>[2x]MEGSEPVAAHQGEEASCSSWGTGSTNKNLPIMSTASVEIDDALYSRQRYVLGDTAMQKMAKSHVFLSGMGGLGLEIAKNLVLAGIKAVTIHDTEKCQAWDLGTNFFLSEDDVVNKRNRAEAVLKHIAELNPYVHVTSSSVPFNETTDLSFLDKYQCVVLTEMKLPLQKKINDFCRSQCPPIKFISADVHGIWSRLFCDFGDEFEVLDTTGEEPKEIFISNITQANPGIVTCLENHPHKLETGQFLTFREINGMTGLNGSIQQITVISPFSFSIGDTTELEPYLHGGIAVQVKTPKTVFFESLERQLKHPKCLIVDFSNPEAPLEIHTAMLALDQFQEKYSRKPNVGCQQDSEELLKLATSISETLEEKPDVNADIVHWLSWTAQGFLSPLAAAVGGVASQEVLKAVTGKFSPLCQWLYLEAADIVESLGKPECEEFLPRGDRYDALR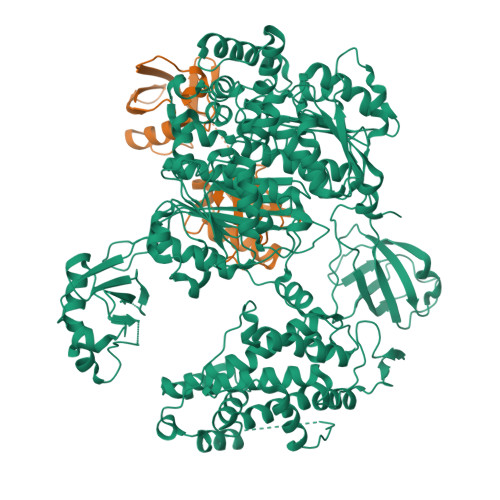ACIGDTLCQKLQNLNIFLVGCGAIGCEMLKNFALLGVGTSKEKGMITVTDPDLIEKSNLNRQFLFRPHHIQKPKSYTAADATLKINSQIKIDAHLNKVCPTTETIYNDEFYTKQDVIITALDNVEARRYVDSRCLANLRPLLDSGTMGTKGHTEVIVPHLTESYNSHRDPPEEEIPIATLKNFPNAIEHTLQWARDEFEGLFKQPAENVNQYLTDPKFVERTLRLAGTQPLEVLEAVQRSLVLQRPQTWADCVTWACHHWHTQYSNNIRQLLHNFPPDQLTSSGAPFWSGPKRCPHPLTFDVNNPLHLDYVMAAANLFAQTYGLTGSQDRAAVATFLQSVQVPEFTPKSGVKIHVSDQELQSANASVDDSRLEELKATLPSPDKLPGFKMYPIDFEKDDDSNFHMDFIVAASNLRAENYDIPSADRHKSKLIAGKIIPAIATTTATVSGLVALEMIKVTGGYPFEAYKNCFLNLAIPIVVFTETTEVRKTKIRNGISFTIWDRWTVHGKEDFTLLDFINAVKEKYGIEPTMVVQGVKMLYVPVMPGHAKRLKLTMHKLVKPTTEKKYVDLTVSFAPDIDGDEDLPGPPVRYYFSHDTD;> TLTVHVRSEEWDLMTFDANPYDSVKKIKEHVRSKTKVPVQDQVLLLGSKILKPRRSLSSYGIDKEKTIHLTLKVVKPSDEELPLFLVESGDEAKRHLLQVRRSSSVAQVKAMIETKTGIIPETQIVTLNGKRLEDGKMMADYGIRKGNLLFLASYSIGG>[6x]AAQPAEALEDDGLCSADQKSCAQSEPDQINEDEFSFKIRRQIEKANADYKPCSSDPQDSDCSCHANVLKRDLAPY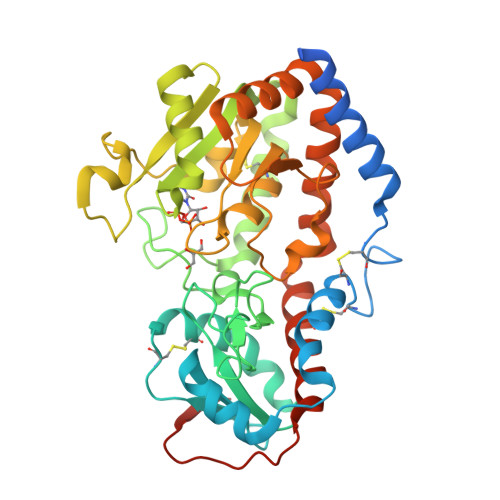KSTGVTRQMIESSARYGTKYKIYGHRLYRDANCMFPARCEGIEHFLLPLVATLPDMDLIINTRDYPQLNAAWGNAAGGPVFSFSKTKEYRDIMYPAWTFWAGGPATKLHPRGIGRWDQMREKLEKRAAAIPWSQKRSLGFFRGSRTSDERDSLILLSRRNPELVEAQYTKNQGWKSPKDTLDAPAADEVSFEDHCKYKYLFNFRGVAASFRLKHLFLCKSLVFHVGDEWQEFFYDQLKPWVHYVPLKSYPSQQEYEHILSFFKKNDALAQEIAQRGYDFIWEHLRMKDIKCYWRKLLKRYVKLLQYEVKPEDQLIYIGPKARALVPR> NVEEETKYIELMIVNDHLMFKKHRLSVVHTNTYAKSVVNMADLIYKDQLKTRIVLVAMETWATDNKFAISENPLITLREFMKYRRDFIKEKSDAVHLFSGSQFESSRSGAAYIGGICSLLKGGGVNEFGKTDLMAVTLAQSLAHNIGIISDKRKLASGECKCEDTWSGCIMGDTGYYLPKKFTQCNIEEYHDFLNSGGGACLFNKPSKLLDPPECGNGFIETGEECDCGTPAECVL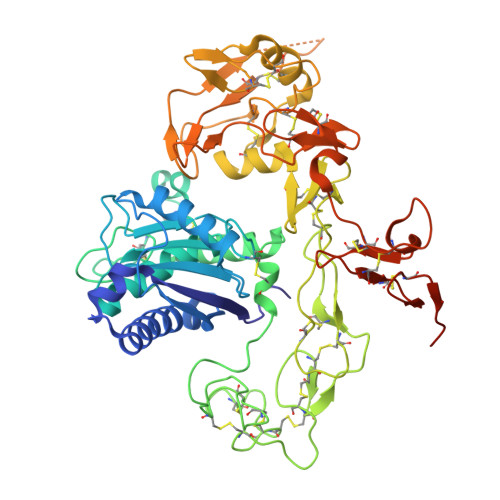EGAECCKKCTLTQDSQCSDGLCCKKCKFQPMGTVCREAVNDCDIRETCSGNSSQCAPNIHKMDGYSCDGVQGICFGGRCKTRDRQCKYIWGQKVTASDKYCYEKLNIEGTEKGNCGKDKDTWIQCNKRDVLCGYLLCTNIGNIPRLGELDGEITSTLVVQQGRTLNCSGGHVKLEEDVDLGYVEDGTPCGPQMMCLEHRCLPVASFNFSTCLSSKEGTICSGNGVCSNELKCVCNRHWIGSDCNTYFPHNDDAKTGITLSGKHHHHHH8-bromanyl-9-(4-bromanylbutyl)purin-6-amine 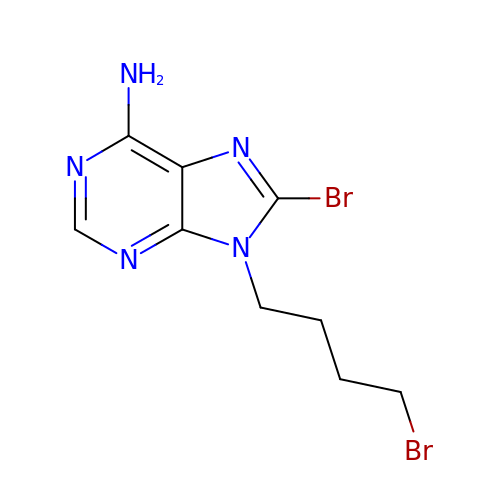| C9 H11 Br2 N5 | VZDKFJGKRZGJKU-UHFFFAOYSA-N>PAFVNKLWSMVNDKSNEKFIHWSTSGESIVVPNRERFVQEVLPKYFKHSNFASFVRQLNMYGWHKVQDVKSGSMLSNNDSRWEFENE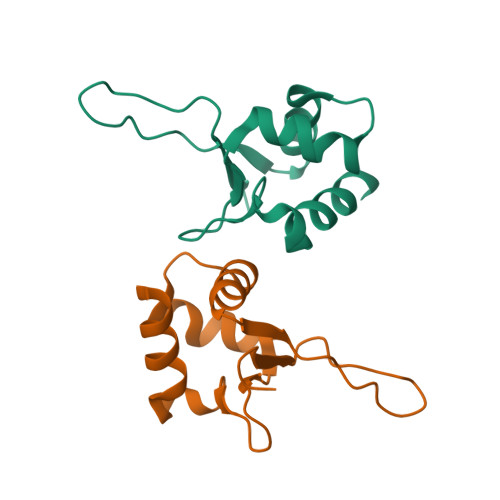RHA[2x]>MHHHHHHENLYFQGRFDNKVVVITGAGNGMGEAAARRFSAEGAIVVLADWAKEAVDKVAASLPKGRAMAVHIDVSDHVAVEKMMNEVAEKLGRIDVLLNNAGVHVAGSVLETSIDDWRRIAGVDIDGVVFCSKFALPHLLKTKGCIVNTASQSGLGGDWGAAYYCAAKGAVVNLTRAMALDHGGDGVRINSVCPSLVKTNMTNGWPQEIRDKFNERIALGR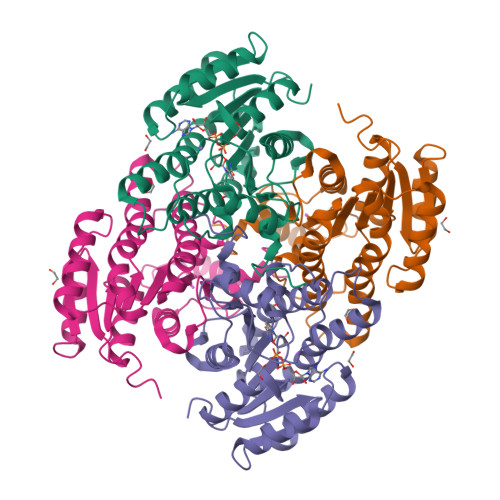AAEPEEVAAVMAFLASDDASFINGANIPVDGGATASDGAPKIV[2x]> MRKPILAALTLAGLGLAQEFITIGSGSTTGVYFPVATGIAKLVNDANVGIRANARSTGGSVANINAINAGEFEMALAQNDIAYYAYQGCCIPAFEGKPVKTIRALAALYPEVVHVVARKDAGIRTVADLKGKRVVVGDVGSGTEQNARQILEAYGLTFDDLGQAIRVSASQGIQLMQDKRADALFYTVGLGASAIQQLALTTPIALVAVDLNRIQAIAKKYPFYVGFNIPGGTYKGVDVTTPTVAVQAMLIASERLSEETVYKFMKAVFGNLEAFKKIHPNLERFFGLEKAVK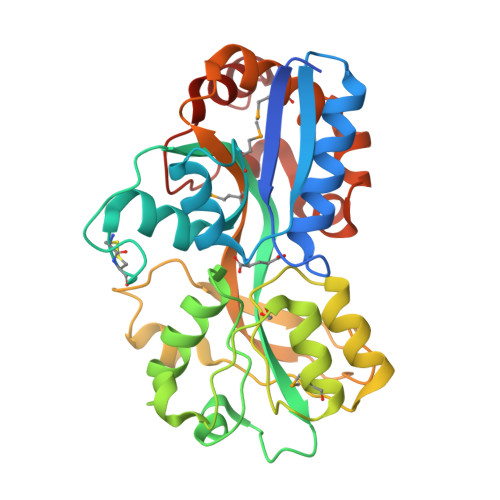GLPIPLHPGAERFYKEAGVLK> GPLGSRRPPREEYSA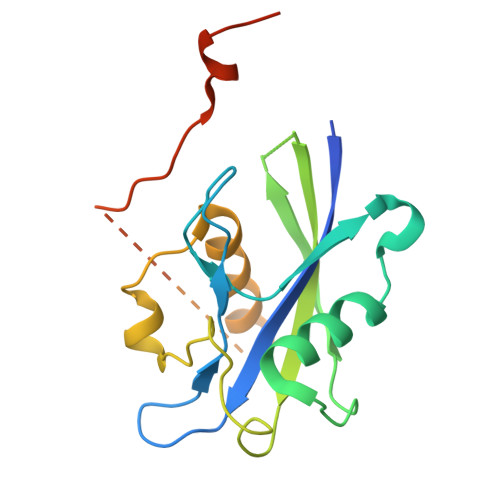TCVVEQPGAIGGPLVLLVQRPDSGLLAGLWEFPSVTLEPSEQHQHKALLQELQRWCGPLPAIRLQHLGEVIHIFSHIKLTYQVYSLALDQAPASTAPPGARWLTWEEFCNAAVSTAMKKVFRMYEDHRQGTRKGSKRSQVCPPSSRKKPSLGQQVLDTFFQRHIPTDKPNSTTQ> MRNLMRCLIMIKSLIKGVDMSRKLAKTRILGYGLMICFLAGCFHPPYNNFQPDRRAVKRVGVDTGIGAVAGAIASGTASGTLIGAAAGGTVGLVASIYRDSKRKIIRDLQKQDIQYVEYGDTRTLIIPTDKYFMFSSPRLNEICYPGLNNVIRLLNFYPQSTIYVAGFTDNVGSRSHKRKLSQAQAETMM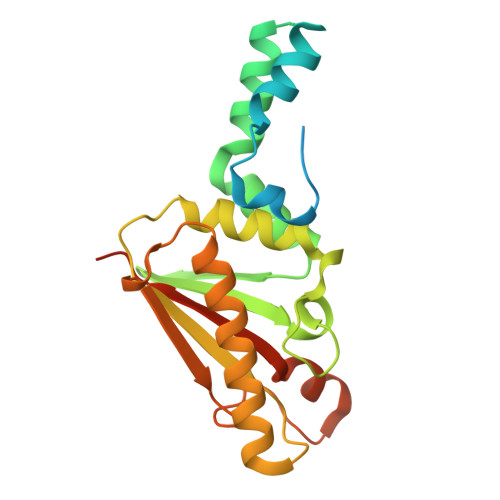TFLWANGIAAKRLKAEGYGDKNAISDNAIIHGSAQNRRIEIQWFTSPAQPPQPQMAYVK>[2x]MASRAPKEVPLCPLMTDGETRNVTDLPGPTNWPLLGSLLEIFWKGGLKKQHDTLAEYHKKYGQIFRMKLGSFDSVHLGSPSLLEALYRTESAHPQRLEIKPWKAYRDHRNEAYGLMILEGQEWQRVRSA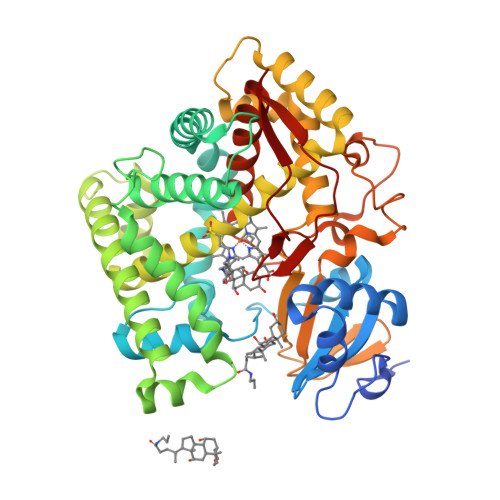FQKKLMKPVEIMKLDKKINEVLADFLERMDELCDERGRIPDLYSELNKWSFESICLVLYEKRFGLLQKETEEEALTFITAIKTMMSTFGKMMVTPVELHKRLNTKVWQAHTLAWDTIFKSVKPCIDNRLQRYSQQPGADFLCDIYQQDHLSKKELYAAVTELQLAAVETTANSLMWILYNLSRNPQAQRRLLQEVQSVLPDNQTPRAEDLRNMPYLKACLKESMRLTPSVPFTTRTLDKPTVLGEYALPKGTVLTLNTQVLGSSEDNFEDSHKFRPERWLQKEKKINPFAHLPFGIGKRMCIGRRLAELQLHLALCWIIQKYDIVATDNEPVEMLHLGILVPSRELPIAFRPR Bilin 584 (doubly linked) | C33 H40 N4 O6 | 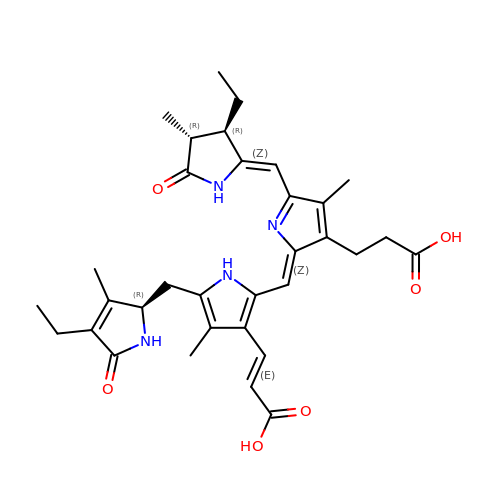KXOMFZIVZHIPRO-GUEBWASOSA-N> GSHMMEAILNKNMKILIVDDFSTMRRIVKNLLRDLG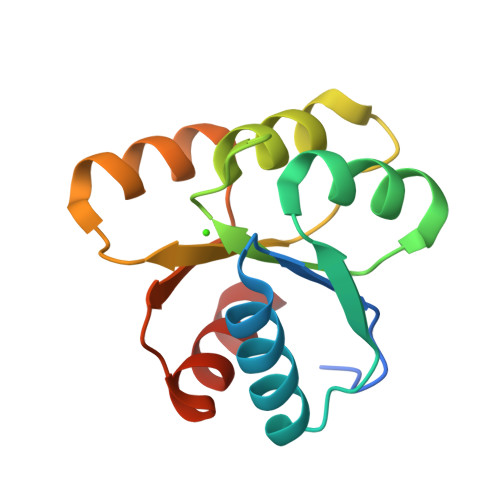FNNTQEADDGLTALPMLKKGDFDFVVTDWNMPGMQGIDLLKNIRADEELKHLPVLMITAEAKREQIIEAAQAGVNGYIVKPFTAATLKEKLDKIFERL>MTNVADIEAANAQYAAAFTKGHLPGPPKRKLAVVTCMDARIDVFSVLGLTEGDAHVIRNAGGRASEALRSLIISQRLGGTEEVVVIHHTDCGMLTFSDEDIRAKIREELGEDASDIKFLPFRDLEASVREDVRFLRGSRLVQG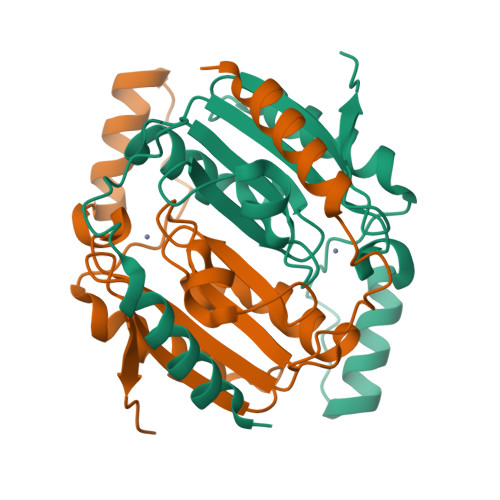NVTGYVYEVERGRLVRLDVSD[2x]>MGHHHHHHHHHHSSGHIEGRHMMAERKGTAKVDFLKKIEKEIQQKWDTERVFEVNASNLEKQTSKGKYFVTFPYPYMNGRLHLGHTFSLSKCEFAVGYQRLKGKCCLFPFGLHCTGMPIKACADKLKREIELYGCPPDFPDEEEEEEETSVKTEDIIIKDKAKGKKSKAAAKAG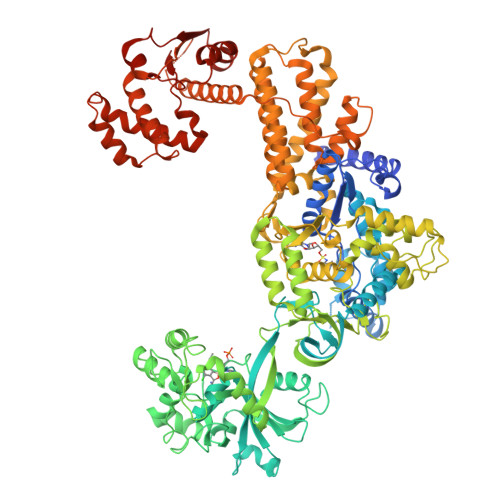SSKYQWGIMKSLGLSDEEIVKFSEAEHWLDYFPPLAIQDLKRMGLKVDWRRSFITTDVNPYYDSFVRWQFLTLRERNKIKFGKRYTIYSPKDGQPCMDHDRQTGEGVGPQEYTLLKLKVLEPYPSKLSGLKGKNIFLVAATLRPETMFGQTNCWVRPDMKYIGFETVNGDIFICTQKAARNMSYQGFTKDNGVVPVVKELMGEEILGASLSAPLTSYKVIYVLPMLTIKEDKGTGVVTSVPSDSPDDIAALRDLKKKQALRAKYGIRDDMVLPFEPVPVIEIPGFGNLSAVTICDELKIQSQNDREKLAEAKEKIYLKGFYEGIMLVDGFKGQKVQDVKKTIQKKMIDAGDALIYMEPEKQVMSRSSDECVVALCDQWYLDYGEENWKKQTSQCLKNLETFCEETRRNFEATLGWLQEHACSRTYGLGTHLPWDEQWLIESLSDSTIYMAFYTVAHLLQGGNLHGQAESPLGIRPQQMTKEVWDYVFFKEAPFPKTQIAKEKLDQLKQEFEFWYPVDLRVSGKDLVPNHLSYYLYNHVAMWPEQSDKWPTAVRANGHLLLNSEKMSKSTGNFLTLTQAIDKFSADGMRLALADAGDTVEDANFVEAMADAGILRLYTWVEWVKEMVANWDSLRSGPASTFNDRVFASELNAGIIKTDQNYEKMMFKEALKTGFFEFQAAKDKYRELAVEGMHRELVFRFIEVQTLLLAPFCPHLCEHIWTLLGKPDSIMNASWPVAGPVNEVLIHSSQYLMEVTHDLRLRLKNYMMPAKGKKTDKQPLQKPSHCTIYVAKNYPPWQHTTLSVLRKHFEANNGKLPDNKVIASELGSMPELKKYMKKVMPFVAMIKENLEKMGPRILDLQLEFDEKAVLMENIVYLTNSLELEHIEVKFASEAEDKIREDCCPGKPLNVFRIEPGVSVS[2x]> MRLLYLHADRFEYKTVKPALKNPPDPPGEASFGEALVVFTTVEDGDGPQTVMYAASDIASHSSRLKVTTVILYPYAHLSSRLAKPMAAHKRLIELEGALRTKFPGHVHRAPFGWYKSFSIACKGHPLAALSRSFTE

We have been interested in a D-aminoacyl-tRNA deacylase (DTD) fold that is present across the domains of life in two different functional contexts: as an N-terminal editing domain (NTD) of archaeal ThrRS, which specifically removes non-cognate L-serine mischarged on tRNAThr, and as a freestanding ‘chiral proofreading' enzyme, which removes D-amino acids from tRNAs in bacteria and eukaryotes. Both share a striking structural and mechanistic similarity highlighting a common ancestry. Here we show, with the help of structural, biochemical and biophysical studies from three distant organisms, that the substrate specificity in this domain is determined by a differential remodelling of the catalytic centre at the RNA–protein interface rather than just the presence or absence of catalytic water as previously proposed. While demonstrating that the tRNA provides the catalytic group, we show that the side chains within the recognition site are dispensable for the proofreading function, suggesting a primordial mode of protein- or peptide scaffold-based enzymatic activity evolved alongside that of RNA.

To rule out any genus-related phenomenon and to test the universality of the observation, we chose to do biochemical experiments with NTD from Aeropyrum pernix (ApNTD), which belongs to a different phylum (Crenarchaeota), and shares ∼43% identity with PabNTD. Remarkably, the corresponding mutants Y115A, E129A and Y115A/E129A in ApNTD also retained completely the capability to discriminate between seryl and threonyl substrates. However, in ApNTD, it has only a water-mediated interaction with the corresponding Glu129, whereas in the case of MjNTD, this group is directly recognized by both Glu135 and His84. Structural studies were also carried out with the mutants of the amino-acid pocket in ApNTD. While E129A mutant also showed a loosening of interactions upon L-Thr3AA binding as observed in the case of wild type, no such loosening was observed in the case of Y115A, thus providing a rationale for rejecting the cognate substrate in the mutants.>[2x]AKQKKEKVWAHYEEQPVEEVMPVLEEKERSASYKPVFVTEITDDLHFYVQDVETGTQLEKLMENMRNDIASHPPVEGSYAPRRGEFCIAKFVDGEWYRARVEKVESPAKIHVFYIDYGNREVLPSTRLGTLSPAFSTRVLPAQATEYAFAFIQVPQDDDARTDAVDSVVRDIQNTQCLLNVEHLSAGCPHVTLQ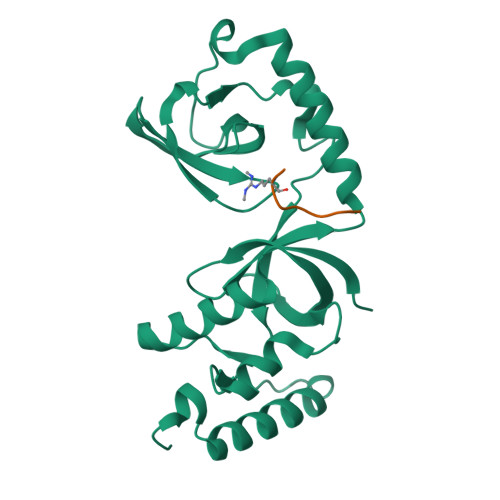FADSKGDVGLGLVKEGLVMVEVRKEKQFQKVITEYLNAQESAKSARLNLWRYGDFRADDADEFGYSR;>TGRARARA[2x]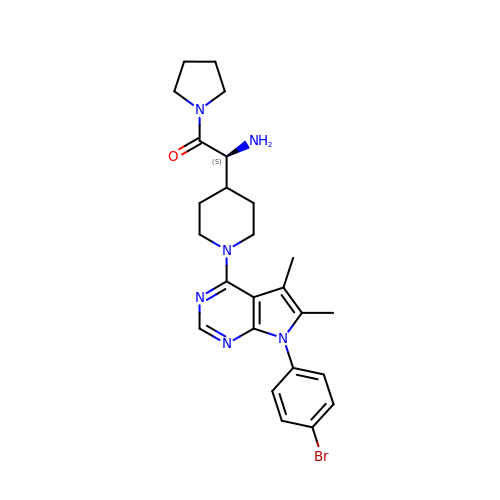(2S)-2-amino-2-{1-[7-(4-bromophenyl)-5,6-dimethyl-7H-pyrrolo[2,3-d]pyrimidin-4-yl]piperidin-4-yl}-1-(pyrrolidin-1-yl)ethan-1-one | C25 H31 Br N6 O | TVTOXROCVZMGPW-QFIPXVFZSA-N> NPVENYIDEVLNEVLVVPNINSSNPTTSNSAPALDAAETGHTSSVQPEDVIETRYVQTSQTRDEMSLESFLGRSGCIHESKLEVTLANYNKENFTVWAINLQEMAQIRRKFELFTYTRFDSEITLVPCISALSQDIGHITMQYMYVPPGAPVPNSRDDYAWQSGTNASVFWQHGQAYPRFSLPFLSVASAYYMFYDGYDEQDQNYGTANTNNMGSLCSRIVTEKHIHKVHIMTRIYHKAKHVKAWCPRPPRALEYTRAHRTNFKIEDRSIQTAIVTRPIITTAGPSDMY;> SPTVEACGYSDRIIQITRGDSTITSQDVANAIVAYGVWPHYLSSKDASAIDKPSQPDTSSNRFYTLRSVTWSSSSKGWWWKLPDALKDMGIFGENMFYHYLGRSGYTIHVQCNASKFHQGTLIVALIPEHQIASALHGNVNVGYNYTHPGETGREVKAETRLNPDLQPTEEYWLNFDGTLLGNITIFPHQFINLRSNNSATIIAPYVNAVPMDSMRSHNNWSLVIIPICPLETSSAINTIPITISISPMCAEFSGARAKRQ;> GLPVFITPGSGQFLTTDDFQSPCALPWYHPTKEISIPGEVKNLVEICQVDSLVPINNTDTYINSENMYSVVLQSSINAPDKIFSIRTDVASQPLATTLIGEISSYFTHWTGSLRFSFMFCGTANTTVKLLLAYTPPGIAEPTTRKDAMLGTHVIWDVGLQSTISMVVPWISASHYRNTSPGRSTSGYITCWYQTRLVIPPQTPPTARLLCFVSGCKDFCLRMARDTNLHLQSGAIAQ

Like all members of the Picornaviridae family, HRVs consist of a T = 1 (pseudo T = 3) icosahedral capsid of about 30 nm in diameter that is built from 60 copies of each of 4 coat proteins VP1, VP2, VP3, and VP4, protecting a plus-sense single-stranded RNA genome. In HRV2, a member of the minor group HRVs, upon binding to lipoprotein receptors (LDL-R) on the cell surface virions are taken up into vesicles and directed to early endosomes. The low pH conditions found in the endosome, and not the binding to LDL-R, catalyze the delivery of the viral genome. After release of the RNA, empty capsids (B-particles) sedimenting at 80S appear and polyprotein synthesis commences.

Here we report the 3.0 Å resolution crystal structure of the HRV2 empty particle. Analysis of the electron density confirmed the absence of VP4, as predicted from comparison with the poliovirus uncoating scenario and the cryo-EM structure of HRV2 previously determined at 15 Å. Externalization of N-terminal residues of VP1 in the empty capsid is compatible with the lack of ordered electron density up to position 1062 (VP1, VP2 and VP3 proteins are numbered starting with 1000, 2000 and 3000 respectively). When compared with the corresponding 314 Å diameter of the native virions, this implies an average expansion of 3.8%, which is in accordance with the observations derived from electron microscopy studies for this virus and other related picornavirus particles. Thus, the rearrangement of VP1 in the 80S empty capsid with respect to the native virion can be explained by a hinge-type movement, consisting in an approximately 5.6° outward rotation of one of these two regions with respect to the other. However, in the 80S particle these subunits are displaced with regard to the VP1 ß-barrel by between 4 and 6 Å towards the icosahedral three-fold axis. In the structure of the 80S particle, the density within the pocket is absent and the cavity appears collapsed. Surprisingly, the 80S empty particle possesses pores or breaks crossing the capsid shell. These pores, absent in the HRV2 native virions, connect the canyon floor with the internal surface of the particle, close to residues Arg1062-Glu1068. Altogether, these changes disrupt 13 interactions of the native capsid and produce a break in the interface between pentamers that crosses the capsid along the two-fold symmetry axes.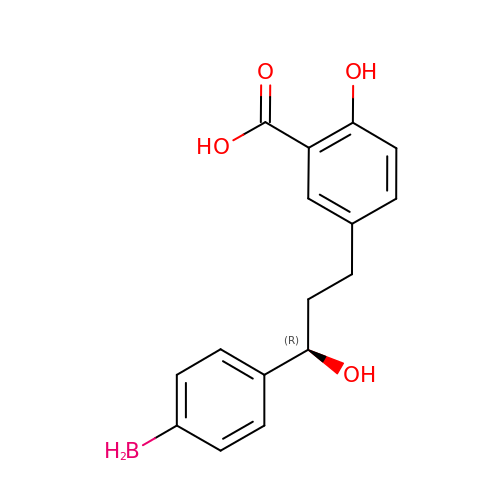5-[(3R)-3-(4-boranylphenyl)-3-oxidanyl-propyl]-2-oxidanyl-benzoic acid | C16 H17 B O4 | AIYINTRBIVHQTG-CQSZACIVSA-N> MYWVRRKTIGGSGLPYTENEILEWRKEG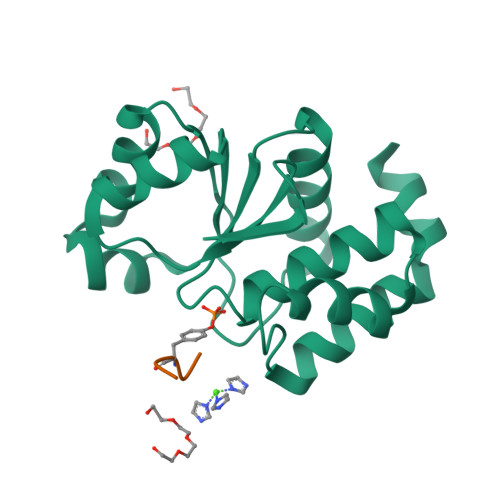VKRVLVLPEDWEIEESWGDKDYYLSILKKNGLQPLHIPIPDGGVPSDSQFLTIMKWLLSEKEGNLVHSVGGIGRTGTILASYLILTEGLEVESAIDEVRLVRPGAVQTYEQEMFLLRVEGMRKSWLKNIYSNS;> NKYGN Some Gram-negative bacteria target their competitors by exploiting the type VI secretion system to extrude toxic effector proteins. To prevent self-harm, these bacteria also produce highly specific immunity proteins that neutralize these antagonistic effectors. The opportunistic pathogen Serratia marcescens has recently been shown to utilize T6-dependent secretion of two family 4 amidases, Ssp1 and Ssp2, to mediate antibacterial activity. In S. marcescens, the resistance-associated proteins Rap1a and Rap2a neutralize Ssp1 and Ssp2, respectively.

Isomorphous crystal structures of Ssp1 (at 1.85 Å resolution) and the active-site Ssp1-C50A mutant (at 2.2 Å resolution) reveal the overall enzyme structure and details of the active site. The protein is a monomer in solution but crystallized with two molecules in the asymmetric unit, each consisting of residues 1–163. The primary, secondary and tertiary structure of Ssp1 classifies it into the NlpC/P60 cysteine peptidase superfamily. An N-terminal subdomain comprises residues 1–95 and is formed by six α-helices (α1–α6) and, on the surface of the protein, a β-hairpin-like loop (β1, turn, β2). A short peptide segment links α6 to β3, which represents the start of the C-­terminal subdomain. This subdomain is dominated by a four-stranded antiparallel β-sheet with order β3–β7–β4–β5, which is flanked on one side by α7 and β6 and on the other by α6. A disulfide bond is observed between Cys146 at the C-­terminal end of β6 and Cys150 located on the loop linking β6 to β7. A cleft, the substrate-binding site, is created between the subdomains by residues in the α1–α2 and α4–α5 links, the C-terminal segment of β6 and the loop leading to β7. Cys50 donates a hydrogen bond to a water molecule, which in turn interacts with His133, Asn48 and Tyr129. Asp135 accepts a hydrogen bond from His133 and appears to complete a catalytic triad reminiscent of that observed in typical cysteine peptidases. The differences evident from structural comparisons suggest that a distinctive and more open substrate-binding surface in Ssp1 compared with those observed in Tae4 structures or implied in Ssp2 might explain the promiscuous endopeptidase activity of Ssp1.

>MKPLYRQLKSSHYSSDYSSPGYLAAEAVYAEIGYELDTLLKQNPGYANTCAVRMSLALLKTGISFKGRLPIKKGAYKGKTIEPGAKLLADQLHRSSSFGKAKIFFNAPDAEKGIGNKKGVVFFNKITNYDGGHIDLIEPENSLLTCHSHCYFNCKEVWFWELS[2x]>[4x]GFPLITITVRGRNVHMKQEHYMKGSDGAPDTGYLWHVPLTFITSKSDMVHRFLLKTKTDVLILPEEVEWIKFNVGMNGYYIVHYEDDGWDSLTGLLKGTHTAVSSNDRASLINNAFQLVSIGKLSIEKALDLSLYLKHETEIMPVFQG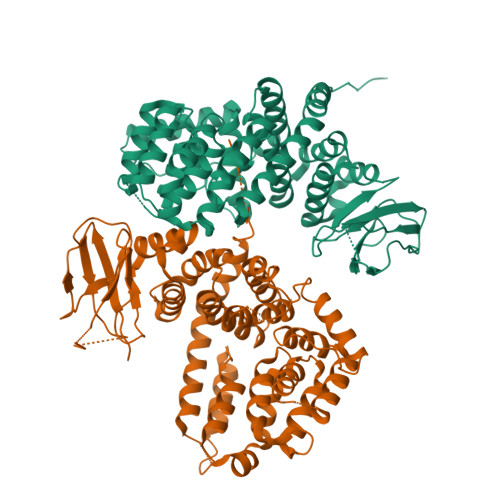LNELIPMYKLMEKRDMNEVETQFKAFLIRLLRDLIDKQTWTDEGSVSERMLRSQLLLLACVHNYQPCVQRAEGYFRKWKESNGNLSLPVDVTLAVFAVGAQSTEGWDFLYSKYQFSLSSTEKSQIEFALCRTQNKEKLQWLLDESFKGDKIKTQEFPQILTLIGRNPVGYPLAWQFLRKNWNKLVQKFELGSSSIAHMVMGTTNQFSTRTRLEEVKGFFSSLKENGSQLRCVQQTIETIEENIGWMDKNFDKIRVWLQSEKLERMAAAAFKARKF>MGNQDTIIETDNGNSDYETPQPTSFPLEHN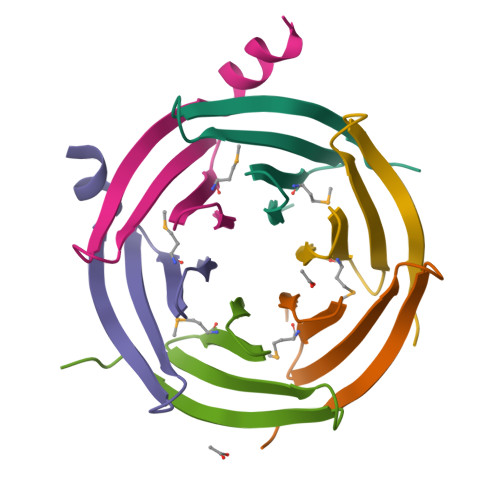HFGVMEDGYIKIYEYNESRNEVKLKKEYADDELELEHHHHHH[6x]> RPNHTIYINNLNEKIKKDELKKSLHA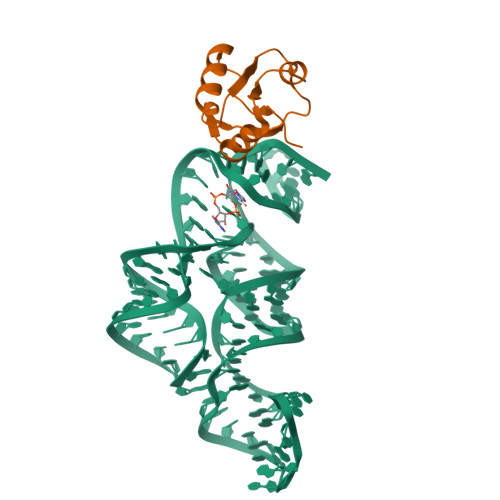IFSRFGQILDILVKRSLKMRGQAFVIFKEVSSATNALRSMQGFPFYDKPMRIQYAKTDSDIIAKMA> MAAHHRQNTAGRRKVQVSYVIRDEVEKYNRNGVNALQLDPALNRLFTAGRDSIIRIWSVNQHKQDPYIASMEHHTDWVNDIVLCCNGKTLISASSDTTVKVWNAHKGFCMSTLRTHKDYVKALAYAKDKELVASAGLDRQIFLWDVNTLTALTASNNTVTTSSLSGNKDSIYSLAMNQLGTIIVSGSTEKVLRVWDPRTCAKLMKLKGHTDNVKALLLNRDGTQCLSGSSDGTIRLWSLGQQRCIATYRVHDEGVWALQVNDAFTHVYSGGRDRKIYCTDLRNPDIRVLICEEKAPVLKMELDRSADPPPAIWVATTKSTVNKWTLKGIHNFRASGDYDNDCTNPITPLCTQPDQVIKGGASIIQCHILNDKRHILTKDTNNNVAYWDVLKACKVEDLGKVDFEDEIKKRFKMVYVPNWFSVDLKTGMLTITLDESDCFAAWVSAKDAGFSSPDGSDPKLNLGGLLLQALLEYWPRTHVNPMDEEENEVNHVNGEQENRVQKGNGYFQVPPHTPVIFGEAGGRTLFRLLCRDSGGETESMLLNETVPQWVIDITVDKNMPKFNKIPFYLQPHASSGAKTLKKDRLSASDMLQVRKVMEHVYEKII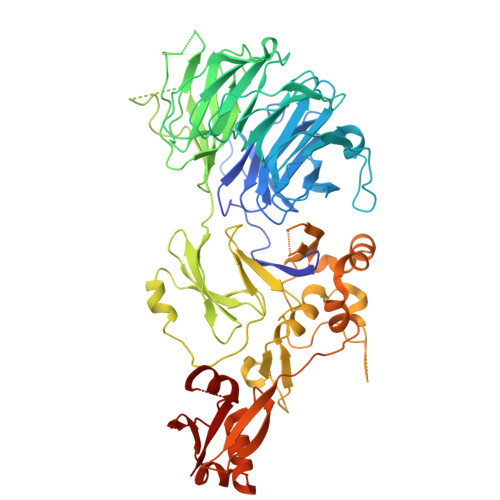NLDNESQTTSSSNNEKPGEQEKEEDIAVLAEEKIELLCQDQVLDPNMDLRTVKHFIWKSGGDLTLHYRQKST> MSEPIDILIAGAGIGGLSCALALHQAGIGKVTLLESSSEIRPLGVGINIQPAAVEALAELGLGPALAATAIPTHELRYIDQSGATVWSEPRGVEAGNAYPQYSIHRGELQMILLAAVRERLGQQAVRTGLGVERIEERDGRVLIGARDGHGKPQALGADVLVGADGIHSAVRAHLHPDQRPLSHGGITMWRGVTEFDRFLDGKTMIVANDEHWS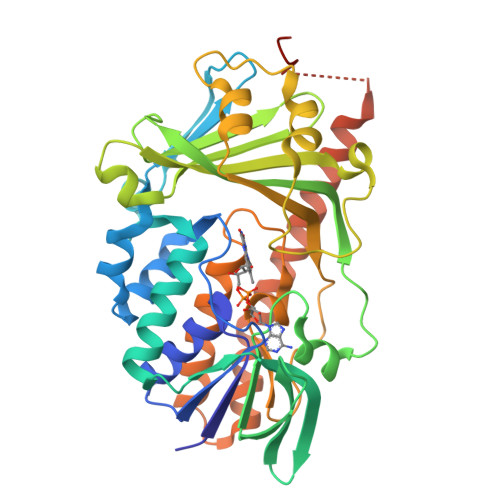RLVAYPISARHAAEGKSLVNWVCMVPSAAVGQLDNEADWNRDGRLEDVLPFFADWDLGWFDIRDLLTRNQLILQYPMVDRDPLPHWGRGRITLLGDAAHLMYPMGANGASQAILDGIELAAALARNADVAAALREYEEARRPTANKIILANREREKEEWAAASRPKTEKSAALEAITGSYRNQVERPRLEHHHHHH> AQVINTNSLSLLTQNNLNKSQSALGTAIERLSSGLRINSAKDDAAGQAIANRFTANIKGLTQASRNANDGISIAQTTEGALNEINNNLQRVRELAVQSANSTNS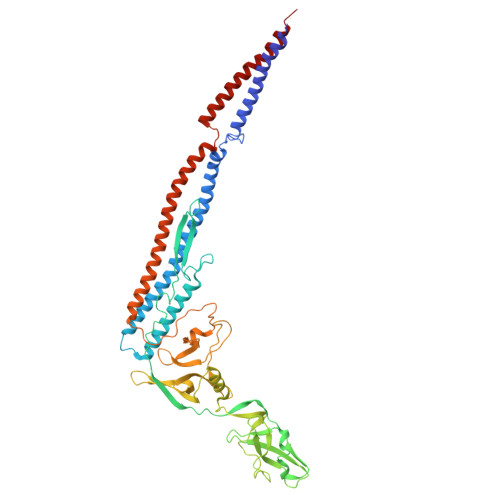QSDLDSIQAEITQRLNEIDRVSGQTQFNGVKVLAQDNTLTIQVGANDGETIDIDLKQINSQTLGLDTLNVQQKYKVSDTAATVTGYADTTIALDNSTFKASATGLGGTDQKIDGDLKFDDTTGKYYAKVTVTGGTGKDGYYEVSVDKTNGEVTLAGGATSPLTGGLPATATEDVKNVQVANADLTEAKAALTAAGVTGTASVVKMSYTDNNGKTIDGGLAVKVGDDYYSATQNKDGSISINTTKYTADDGTSKTALNKLGGADGKTEVVSIGGKTYAASKAEGHNFKAQPDLAEAAATTTENPLQKIDAALAQVDTLRSDLGAVQNRFNSAITNLGNTVNNLTSVRSRIEDSDYATEVSNMSRAQILQQAGTSVLAQANQVPQNVLSLLR> MSELFGVLKSNAGRIILKDPSATSKDVKAYID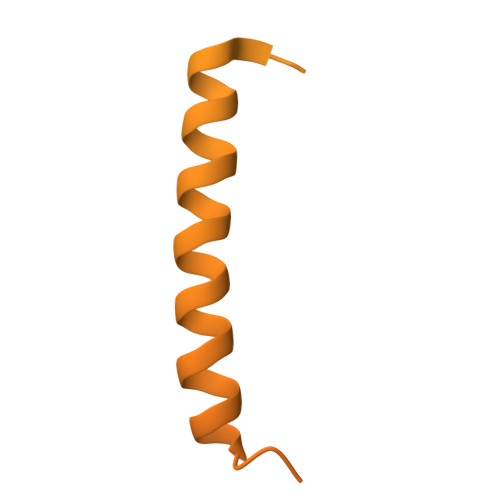SVINTCKNGSITKKAELDEITVDGLDANQVWWQVKLVLDSIDGDLIQGIQELKDVVTPSHNLSDGSTLNSSSGEESELEEAESVFKEKQMLSADVSEIEEQSNDSLSENDEEPSMDDEKTSAEAAREEFAEEKRISSGQDERHSSPDPYGINDKFFDLEKFNRDTLAAEDSNEASEGSEDEDIDYFQDMPSDDEEEEAIYYEDFFDKPTKEPVKKHSDVKDPKEDEELDEEEHDSAMDKVKLDLFADEEDEPNAEGVGEASDKNLSSFEKQQIEIRKQIEQLENEAVAEKKWSLKGEVKAKDRPEDALLTEELEFDRTAKPVPVITSEVTESLEDMIRRRIQDSNFDDLQRRTLLDITRKSQRPQFELSDVKSSKSLAEIYEDDYTRAEDESALSEELQKAHSEISELYANLVYKLDVLSSVHFVPKPASTSLEIRVETPTISMEDAQPLYMSNASSLAPQEIYNVGKAEKDGEIRLKNGVAMSKEELTREDKNRLRRALKRKRSKANLPNVNKRSKRNDVVDTLSKAKNITVINQKGEKKDVSGKTKKSRSGPDSTNIKL> GPKVPESGSMNLAAAERKKTGDLSVRSLHDIVKPEDFVLNSE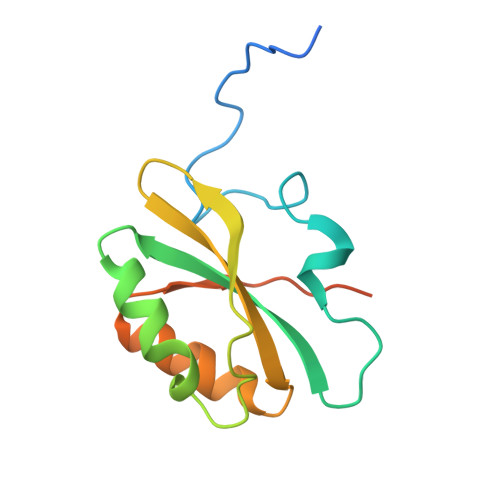HLTTVLVAVPKSLKSDFEKSYETLSKNVVPASASVIAEDAEYVLFNVHLFKKNVQEFTTAAREKKFIPREFNYSEELIDQLKKEHDSA>ASAWPEEKNYHQPAILNSSALRQIAEGTSISEMWQNDLQPLLIERYPGSPGSYAARQHIMQRIQRLQADWVLEIDTFLSQTPYGYRSFSNIISTLNPTAKRHLVLACHYDSKYFSHWNNRVFVGATDAAVPCAMMLELARALDKKLLSLKTVSDSKPDLSLQLIFFDGEEAFLHWSPQDSLYGSRHLAAKMASTP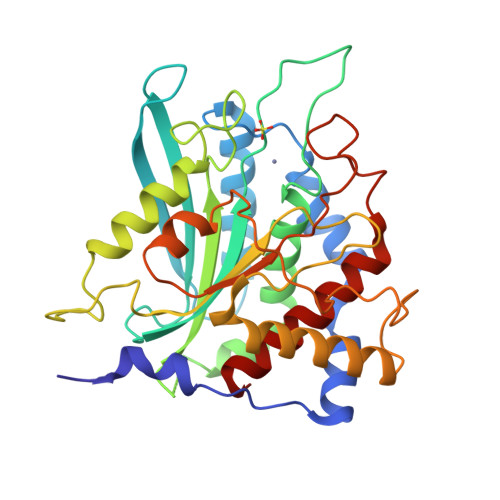HPPGARGTSQLHGMDLLVLLDLIGAPNPTFPNFFPNSARWFERLQAIEHELHELGLLKDHSLEGRYFQNYSYGGVIQDDHIPFLRRGVPVLHLIPSPFPEVWHTMDDNEENLDESTIDNLNKILQVFVLEYLHL[2x]> MAAQGFLLIATFLLVLMVLARPLGSGLARLINDIPLPGTTGVERVLFRALGVSDREMNWKQYLCAILGLNMLGLAVLFFMLLGQHYLPLNPQQLPGLSWDLALNTAVSFVTNTNWQS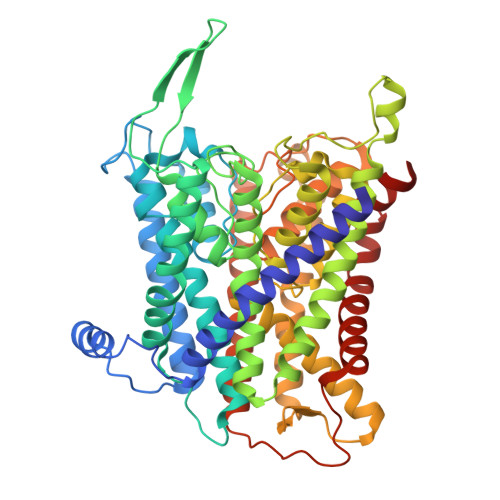YSGETTLSYFSQMAGLTVQNFLSAASGIAVIFALIRAFTRQSMSTLGNAWVDLLRITLWVLVPVALLIALFFIQQGALQNFLPYQAVNTVEGAQQLLPMGPVASQEAIKMLGTNDGGFFNANSSHPFENPTALTNFVQMLAIFLIPTALCFAFGEVMGDRRQGRMLLWAMSVIFVICVGVVMWAEVQGNPHLLALGTDSSINMEGKESRFGVLVSSLFAVVTTAASCGAVIAMHDSFTALGGMVPMWLMQIGEVVFGGVGSGLYGMMLFVLLAVFIAGLMIGRTPEYLGKKIDVREMKLTALAILVTPTLVLMGAALAMMTDAGRSAMLNPGPHGFSEVLYAVSSAANNNGSAFAGLSANSPFWNCLLAFCMFVGRFGVIIPVMAIAGSLVSKKSQAASSGTLPTHGPLFVGLLIGTVLLVGALTFIPALALGPVAEYLS>[6x]MEAVKTDRAPAAIGPYAQAVKAGGFVFVSGQIPLAPDGSLVEGDIRVQTERVMENLKAVLEAAGSGLSRVVQ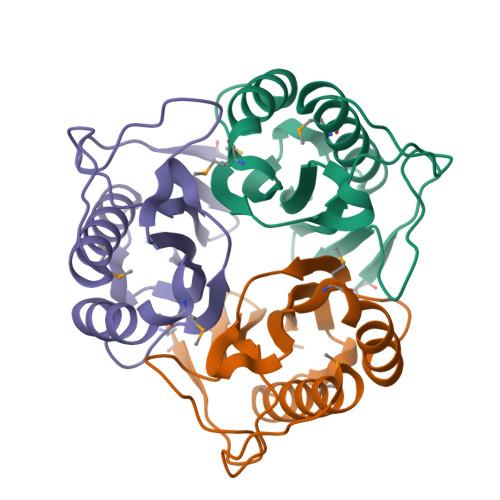TTCFLADMEDFPGFNEVYARYFTPPYPARATVAVKALPRGVRVEVACVALAE> GKTITDFSISRSVLAKYEVINQVDKKFILIR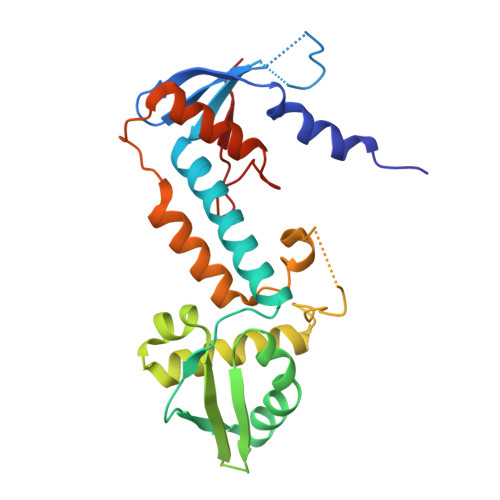CLDQSIHNCPLLVLVDQHACDERIRLEELFYSLLTEVVTGTFVARDLKDCCIEVDRTEADLFKHYQSEFKKWGIGYETIEGTMETSLLEIKTLPEMLTSKYNGDKDYLKMVLLQHAHDLKDFKKLPMDLSHFENYTSVDKLYWWKYSSCVPTVFHEILNSKACRSAVMFGDELTRQECIILISKLSRCHNPFECAHGRPSMVPIAELK> MSSRDLLLKAKENGRKSLLEHEAKYFISSYGIPVTNIRLAKSEEEAVNFSREIGFPVVLKIVSPQVVHKSDVGGVKVNLRSEEEVRKAY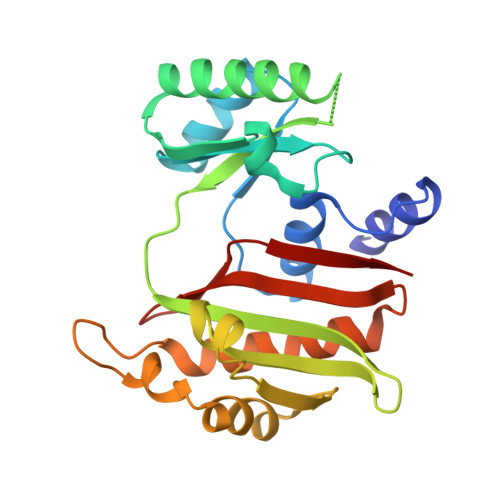REIIENVKRNVPNAEIEGILVQEFAPPGVELIIGLLRDPQFGPTVMFGLGGVFVELFRDVSFRVAPLSEQDAESMIKEVKAYKLLTGFRGMEPVDIEAIKDALIRAGRIGVENEEIAEMDLNPVIAYPKGIKVVDARIILR>MCGIFAYLNYHVPRTRREILETLIKGLQRLEYRGYDSAGVGFDGGNDKDWEANACKIQLIKKKGKVKALDEEVHKQQDMDLDIEFDVHLGIAHTRWATHGEPSPVNSHPQRSDKNNEFIVIHNGIITNYKDLKKFLESKGYDFESETDTETIAKLVKYMYDNRESQDTSFTTLVERVIQQLEGAFALVFKSVHFPGQAVGTRH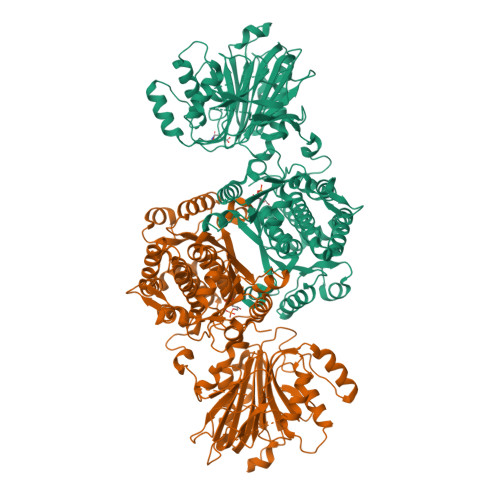GSPLLIGVRSEHKLSTDHIPILYRTGKDKKGSCNLSRVDSTTCLFPVEEKAVEYYFASDASAVIEHTNRVIFLEDDDVAAVVDGRLSIHRIKRTAGHHHHHHDHPGRAVQTLQMELQQIMKGNFSSFMQKEIFEQPESVVNTMRGRVNFDDYTVNLGGLKDHIKEIQRCRRLILIACGTSYHAGVATRQVLEELTELPVMVELASDFLDRNTPVFRDDVCFFLSQSGETADTLMGLRYCKERGALTVGITNTVGSSISRETDCGVHINAGPEIGVASTKAYTSQFVSLVMFALMMCDDRISMQERRKEIMLGLKRLPDLIKEVLSMDDEIQKLATELYHQKSVLIMGRGYHYATCLEGALKIKEITYMHSEGILAGELKHGPLALVDKLMPVIMIIMRDHTYAKCQNALQQVVARQGRPVVICDKEDTETIKNTKRTIKVPHSVDCLQGILSVIPLQLLAFHLAVLRGYDVDFPRNLAKSVTVE[2x]> 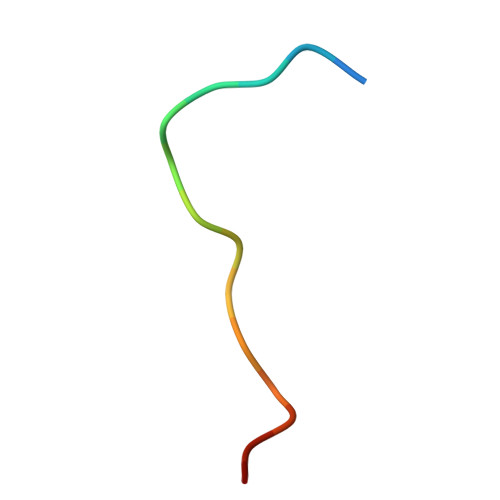RPTPRPVPMKRHIFRS> AMDGTAAEPRPGAGSLQHAQPPPQPRSKRPEDFKFGKILGEGSFSTVVLARELATSREYAIKIVEKRHVNKENKIPYVQREKDVMSRLDHPFFVKLYFCFQDDEKLYFGLSYAKNGELLKYIRKIGSFDETCTRFYTAEIVSALEYLHGKGIIHRDLKPENILLNEDMHIQITDFGTAKVLSPESKQARANSFVGTAQYVSPELLTEKSACKSSDLWALGCIIYQLVAGLPPFRAGNEGLIFAK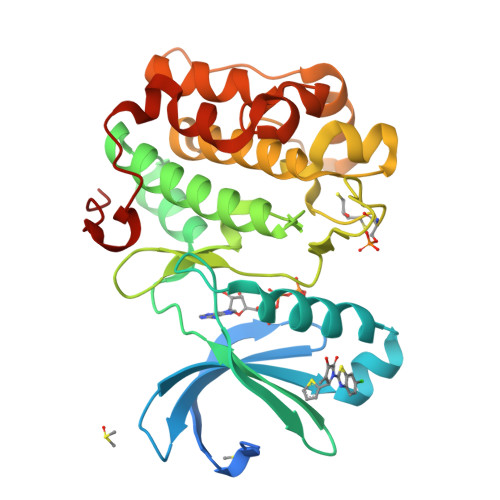IIKLEYDFPEKFFPKARDLVEKLLVLDATKRLGCEEMEGYGPLKAHPFFESVTWENLHQQTPPKLT> MQAVTRFFRHLITLTAVALLAAFLDTVNAAKDTAAGHVTTPCTEILFDLTLAKHYENQIQAAESALNRNYAAIRSWTLLEAMSSDGNRQNAYTGLIAYGIQITVNAEQELQGPKQTKLRAAHALRHRAANLSAALQIQAAQQATLTKPTAGGAQTPFSGATGTCKYEGITATAGEQSCKYSTEDEEKINAAHMNPEVMTQITTIGDKYLTTITLDAIAGSKGNPTQSSATYAEQDCQDGGNPGPNFGGANALGLQVTKLGTKATTEKTNLYTAGGTECEHQPGNGPQKTKQRLAYLVCEANKAAIITPTDLQTLTLDALISAPEMAAIGDALLTDEPATEKEYSSAQHTQIQQLLKKAYGQTNEQFQKNFIKPLAAQTVKFKIGGAEVSNTVAALMSSPNSGLALAYHKGKNKLQHQVKPDTPLVESKKGSECQVIEDK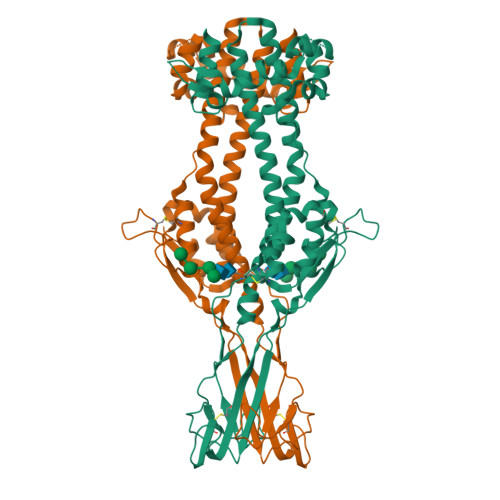EKCKTTYGCELKGDKCVVKMTTKGEVTGTQNTTGSNSFVIKKAPLLLAFLLF> AAVKLAPPTDVRSGYIRL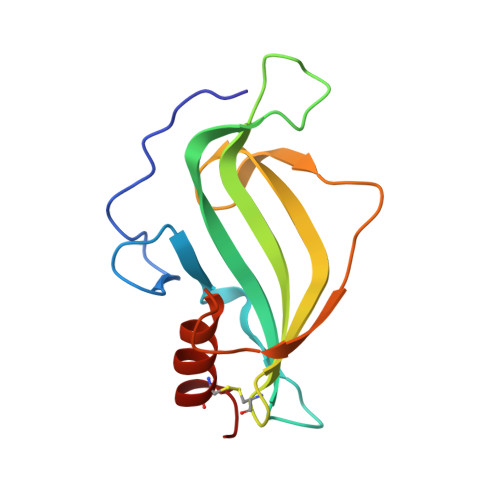VKNVNYYIDSESIWVDNQEPQIVHFDAVVNLDKGLYVYPEPKRYARSVRQYKILNCANYHLTQVRTDFYDEFWGQGLRAAPKKQKKHTLSLTPDTTLYNAAQIICANYGEA> MDPFLVLLHSVSSSLSSSELTELKGLCLGRVGKRKLERVQSGLDLFSMLLEQNDLEPGHTELLRELLASLRRHDLLRRVDDFEAGAAAGAAPGEEDLCAAFNVICDNVGKDWRRLARQLKVSDTKIDSIEDRYPRNLTERVRESLR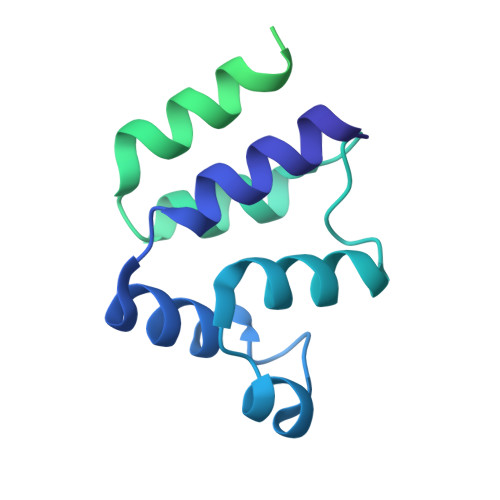IWKNTEKENATVAHLVGALRSCQMNLVADLVQEVQQARDLQNRSGAMSPMSWNSDASTSEASLEHHHHHH>[2x]GSFELSVQDLNDLLSDGSGCYSLPSQPCNEVTPRIYVGNASVAQDIPKLQKLGITHVLNAAEGRSFMHVNTNANFYKDSGITYLGIKA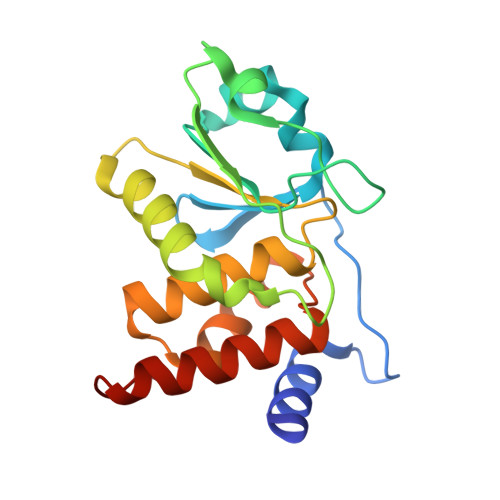NDTQEFNLSAYFERAADFIDQALAQKNGRVLVHCREGYSRSPTLVIAYLMMRQKMDVKSALSIVRQNREIGPNDGFLAQLCQLNDRLAKEGKLKP>[4x]MRGS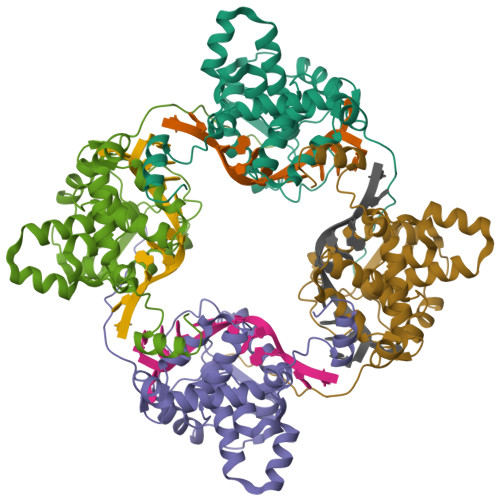HHHHHHGSIEGRIELEFHDVAANTSSTFDPEVAYANFKRVHTTGLSYDHIRIFYIKGREIKTSLAKRSEWEVTLNLGGWKITVYNTNFPGNRNSPVPDDGLTLHRLSGFLARYLLEKMLKVSEPEKLIIKSKIINPLAEKNGITWNDGEEVYLSFFPGSEMFLGTFRFYPLAIGIYKVQRKEMEPKYLEKTMRQRYMGLEAATWTVSKLTEVQSALTVVSSLGWKKTNVSAAARDFLAKFGINM> DEAPADRLKALVDAAVQPVMKANDIPGLAVAISLKGEPHYFSYGLASKEDGRRVTPETLFEIGSVSKTFTATLAGYALAQDKMRLDDRASQHWPALQGSRFDGISLLDLATYTAGGLPLQFPDSVQKDQAQIRDYYRQWQPTYAPGSQRLYSNPSIGLFGYLAARSLGQPFERLMEQQLFPALGLEQTHLDVPEAALAQYAQGYGKDDRPLRVGPGPLDAEGYGVKTSAADLLRFVDANLHPERLDR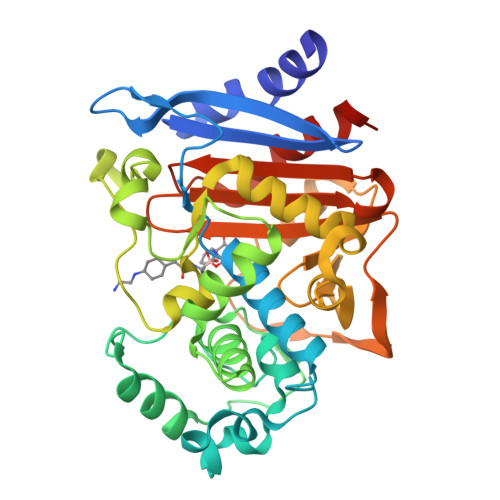PWAQALDATHRGYYKVGDMTQGLGWEAYDWPISLKRLQAGNSMALQPHRIARLPAPQALEGQRLLNKTGSTNGFGAYVAFIPGRDLGLVILANRNYPNAERVKIAYAILSGLEQQAKVPLKR>MKNKKDKGLLSGKLTPAQSKNPAKNELYLVEGDSAGGSAKQGRDRKFQAILPLRGKVINTAKAKMADILKNEEINTMIYTIGAGVGADFSIEDANYDKIIIMTDADTDGAHIQTLLLTFFYRYMRPLVEAGHVYIALPPLYKMSKGKGKKEEVAYAWTDGELEELRKQFGKGATLQRYKGLGEMNADQLWETTMNPETRTLIRVTIEDLARAERRVNVLMGDKVEPRRKWIEDNVKFTLEEATVFHMSNIQNMSLEDIMGERFGRYSKYIIQDRALPDIRDGLKPVQRRILYSMNKDSNTFDKSYRKSAKSVGNIMGNFHPHGDSSIYDAMVRMSQNWKNREILVEMHGNNGSMDGDPPAAMRYTEARLSEIAGYLLQDIEKKTVPFAWNFDDTEKEPTVLPAAFPNLLVNGSTGISAGYATDIPPHNLAEVIDAAVYMIDHPTAKIDKLMEFLPGPDFPTGAIIQGRDEIKKAYETGKGRVVVRSKTEIEKLKGGKEQIVITEIPYEINKANLVKKIDDVRVNNKVAGIAEVRDESDRDGLRIAIELKKDANTELVLNYLFKYTDLQINYNFNMVAIDNFTPRQVGIVPILSSYIAHRREVILARSRFDKEKAEKRLHIVEGLIRVISILDEVIALIRASENKADAKENLKVSYDFTEEQAEAIVTLQLYRLTNTDVVVLQEEEAELREKIAMLAAIIGDERTMYNLMKKELREVKKKFATPRLSSLEDTAKALEHHHHHH[2x]

Delafloxacin is a potent anionic fluoroquinolone approved for the treatment of respiratory infections that acts by trapping the DNA cleavage complexes of bacterial topoisomerase IV and gyrase. Topo IV is a tetrameric complex made up of two ParE and two ParC subunits that mediates unlinking of interlocked daughter chromosomes. Fluoroquinolones stabilise this complex which cellular processes convert into a lethal lesion, likely a frank double-stranded DNA break.

Moreover, a V18 structure solved at an unprecedented 2.0 Å resolution was obtained by improving the crystal quality through seeding with a graphene-PEG nucleant. The PEG chains of the nucleant are thought to attract the complex to the flat and porous graphene surface, creating a localised supersaturated environment favouring protein aggregation. Except for analysis of the drug chelated Mg2+ (which is better defined in the 2.4 Å E-site structure solved by combining multiple data sets), we focus largely on the 2.0 Å V-site structure, whose overall higher resolution meant that the electron densities of the bound drug, the base pairs of the DNA, the puckering of sugars of the DNA, and the side chains and main chain of the protein are generally much better defined as is the water structure. Moreover, we see >1000 individually imaged water molecules including those in the inner and outer co-ordination spheres of the two pairs of functionally distinct magnesium ions, and at a pair of K+ sites discovered here in ParC. In our topo IV-DNA structures, the Mg2+ chelated delafloxacin molecules are bound in a highly unusual conformation in which strikingly the 6-amino-3,5-difluoro-2-pyridinyl substituent at N-1 is tilted 51.2o out-of-plane of the aromatic bicyclic quinolone core. The bulky C-8 chlorine is also out-of-plane by 6.8o and interacts with the face of the adjacent tilted 2-pyridinyl ring at N-1. In this regard, the 2.0 Å delafloxacin complex is highly informative as all six positions in the coordination sphere of the active site Mg2+ ions are clearly resolved. Two of the six inner coordination sites are occupied directly by sidechain carboxyl oxygens from ParE D508 and D506. A third carboxyl oxygen from ParE D433 is linked to the Mg2+ through a clearly visible inner sphere water. The remaining three inner coordination positions are occupied by three water molecules, one of which links to the non-scissile phosphodiester group joining nucleotides at -2 and -1, with a second water potentially bridging to the more distant phosphotyrosyl formed by the catalytic ParC Y118.>[4x]MAKRSLRKMWRPGEKKEPQGVVYEDVPDDTEDFKESLKVVFEGSAYGLQNFNKQKKLKRCDDMDTFFLHYAAAEGQIELMEKITRDSSLEVLHEMDDYGNTPLHCAVEKNQIESVKFLLSRGANPNLRNFNMMAPLHIAVQGMNNEVMKVLLEHRTIDVNLEGENGNTAVIIACTTNNSEALQILLKKGAKPCKSNKWGCFPIHQAAFSGSKECMEIILRFGEEHGYSRQLHINFMNNGKATPLHLAVQNGDLEMIKMCLDNGAQIDPVEKGRCTAIHFAATQGATEIVKLMISSYSGSVDIVNTTDGCHETMLHRASLFDHHELADYLISVGADINKIDSEGRSPLILATASASWNIVNLLLSKGAQVDIKDNFGRNFLHLTVQQPYGLKNLRPEFMQMQQIKELVMDEDNDGCTPLHYACRQGGPGSVNNLLGFNVSIHSKSKDKKSPLHFAASYGRINTCQRLLQDISDTRLLNEGDLHGMTPLHLAAKNGHDKVVQLLLKKGALFLSDHNGWTALHHASMGGYTQTMKVILDTNLKCTDRLDEDGNTALHFAAREGHAKAVALLLSHNADIVLNKQQASFLHLALHNKRKEVVLTIIRSKRWDECLKIFSHNSPGNKCPITEMIEYLPECMKVLLDFCMLHSTEDKSCRDYYIEYNFKYLQCPLEFTKKTPTQDVIYEPLTALNAMVQNNRIELLNHPVCKEYLLMKWLAYGFRAHMMNLGSYCL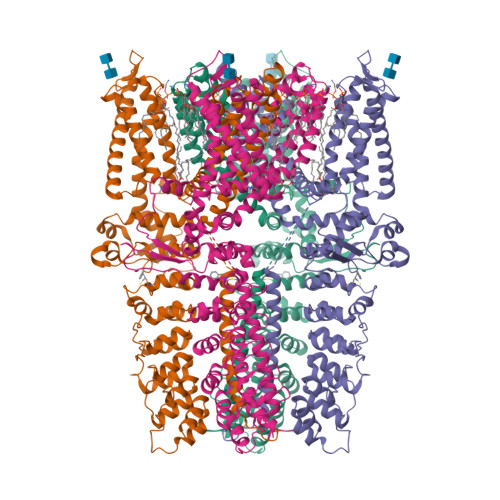GLIPMTILVVNIKPGMAFNSTGIINETSDHSEILDTTNSYLIKTCMILVFLSSIFGYCKEAGQIFQQKRNYFMDISNVLEWIIYTTGIIFVLPLFVEIPAHLQWQCGAIAVYFYWMNFLLYLQRFENCGIFIVMLEVILKTLLRSTVVFIFLLLAFGLSFYILLNLQDPFSSPLLSIIQTFSMMLGDINYRESFLEPYLRNELAHPVLSFAQLVSFTIFVPIVLMNLLIGLAVGDIAEVQKHASLKRIAMQVELHTSLEKKLPLWFLRKVDQKSTIVYPNKPRSGGMLFHIFCFLFCTGEIRQEIPNADKSLEMEILKQKYRLKDLTFLLEKQHELIKLIIQKMEIISETEDDDSHCSFQDRFKKEQMEQRNSRWNTVLRAVKAKTHHLEPSNSLEVLFQGPAADYKDDDDKAHHHHHHHHHH>[2x]GSHMSTEKYHQYKINQPEYKAANGKWEIIEF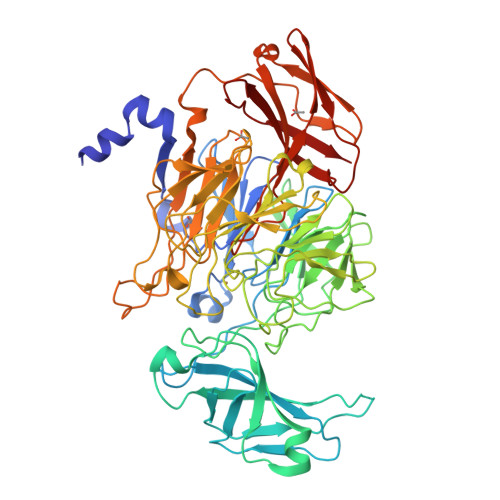PEKYRQNTIHAALLRTGKVLMVAGSGNNQDNSDDKQYDTRIWDPVKGTIKKVPTPSDLFCTGHTQLANGNLLIAGGTKRYEKLKGDVTKAGGLMVVHNENPDKPITLPAGTKFTGKENGKTFVSKDPVLVPRAEKVFDPATGAFVRNDPGLGRIYVEAQKSGSAYETGTEDNYRVQGLSGADARNTYGIAQKLALDKKDFQGIRDAFEFDPVAEKYIKVDPMHEARWYPTLTTLGDGKILSVSGLDDIGQLVPGKNEVYDPKTKAWTYTDKVRQFPTYPALFLMQNGKIFYSGANAGYGPDDVGRTPGVWDVETNKFTKVPGMSDANMLETANTVLLPPAQDEKYMVIGGGGVGESKLSSEKTRIADLKADDPKFVDGPSLEKGTRYPQASILPDDSVLVSGGSQDYRGRGDSNILQARLYHPDTNEFERVADPLVGRNYHSGSILLPDGRLMFFGSDSLYADKANTKPGKFEQRIEIYTPPYLYRDSRPDLSGGPQTIARGGSGTFTSRAASTVKKVRLIRPSASTHVTDVDQRSIALDFKADGDKLTVTVPSGKNLVQSGWYMMFVTDGEGTPSKAEWVRVP> SMATRFMTDPHAMRDMAGRFEVHAQTVEDEARRMWASAQNISGAGWSGMAEATSLDTMAQMNQA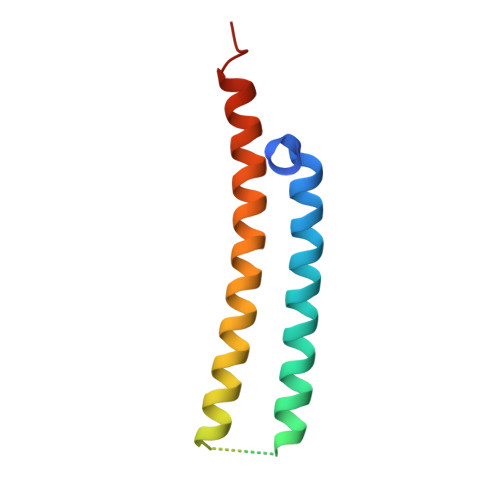FRNIVNMLHGVRDGLVRDANNYEQQEQASQQILSS(2~{S},3~{S},4~{R},5~{R},6~{R})-4,5-diacetamido-6-[[[(2~{R},3~{S},4~{R},5~{R})-5-[2,4-bis(oxidanylidene)pyrimidin-1-yl]-3,4-bis(oxidanyl)oxolan-2-yl]methoxy-oxidanyl-phosphoryl]oxy-oxidanyl-phosphoryl]oxy-3-oxidanyl-oxane-2-carboxylic 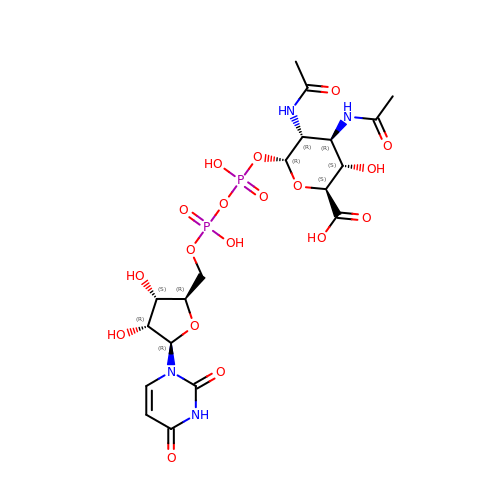acid | C19 H28 N4 O18 P2 | GZLIMKLKXDFTJR-LTMKHLKMSA-N>SNAMSFRIGHGYDVHKFTSAKQNIIIGGVEIAYHLGLEAHSDGDVLIHALCDAILGALGLGDIGKHFLDTDNQFKNIDSKFFLAEIKKMLDKKQYSIS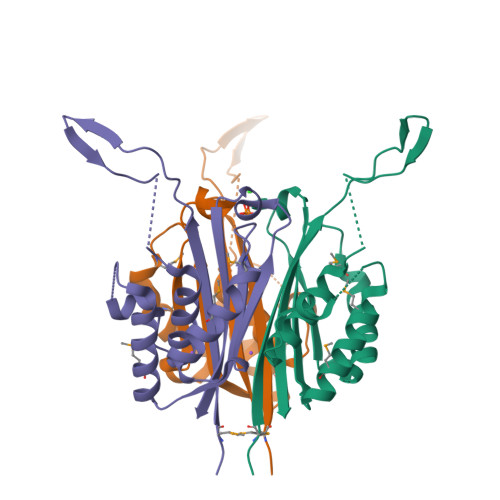NIDCTIIAQAPKMLPHIEKMRACLANILEIQISQINIKATTTERLGFIGREEGIATHVVCLLYR[4x]N-TETRAZOL-5-YL 9-OXO-9H-XANTHENE-2 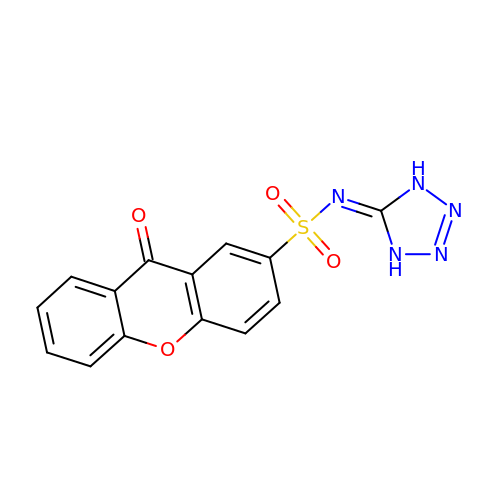SULPHONAMIDE | C14 H9 N5 O4 S | HJWYZPGYPZNDTN-UHFFFAOYSA-N>QTGGSFYEPFNNYNTGLWQKWAFDHVSMTSLGEMRLSLTSPSYNKFDGGGNQSVQTYGYGLYEVNMKPAKNVGIVSAFYTSTGPTDGTPWDEIDIEFLGKDTTKVQFNYYTNGVGNHEKIVNLGFDAANSYHTYAFDWQPNSIKWYVDGQLKHTATTQIPQTPGKIYMSLWAGAGVDEWLGSYNGVTPLYAHYNWVRYTKR[2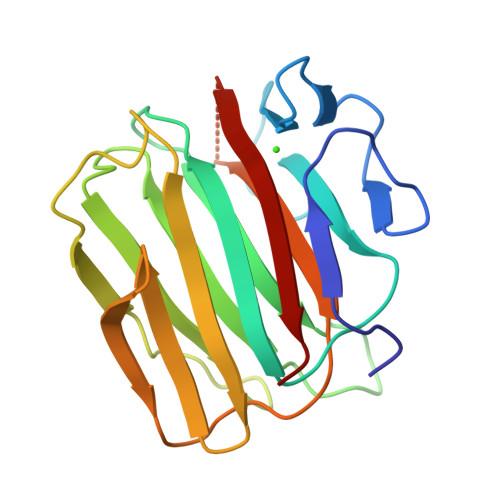x]>[3x]MPFITVGQENSTSIDLYYEDHGTGVPVVLIHGFPLSGHSWERQSAALLDAGYRVITYDRRGFGQSSQPTTGYDYDTFAADLNTVLETLDLQDAVLVGFSMGTGEVARYVSSYGTARIAAVAFLASLEPFLLKTDDNPDGAAPQEFFDGIVAAVKADRYAFYTGFFNDFYNLDENLGTRISEEAVRNSWNTAASGGFF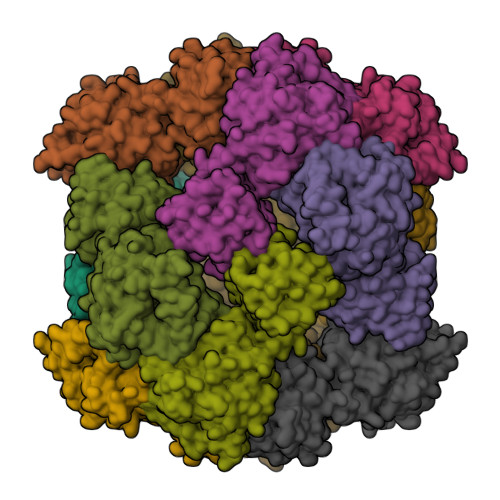AAAAAPTTWYTDFRADIPRIDVPALILHGTGDRTLPIENTARVFHKALPSAEYVEVEGAPHGLLWTHAEEVNTALLAFLAKALEAQKQKLLTEVETYVLSIIPSGPLKAEIAQRLEDVFAGKNTDLEVLMEWLKTRPILSPLTKGILGFVFTLTVPSERGLQRRRFVQNALNGNGDPNNMDKAVKLYRKLKREITFHGAKEISLSYSAGALASCMGLIYNRMGAVTTEVAFGLVCATCEQIADSQHRSHRQLEHHHHHH>[3x]MDTKGRLVAGSHNRNEFVLINADETARVAVTELSGQICQICGDELEVTVNGEPFVACNECAFPVCRPCYEYERREGNQVCPQCKTRYKRIKGSPRVEGDEEEDDSDDLESEFDIGSVFSARLNYGSQVNGSVIHAPSEFDAASVASEIPLLTYGQEDVGISADKHALILPPFTARGKRVHPMPFPDSSVPVQPRPMDPKKDIAVYGYGSVAWKERMEDWKKKQSEKLQVVRHEGGKDSDELDDPDLPKMDEGRQPLWRKLPISSSRINPYRIIIVLRIAILCLFFHYRILHPVNDAYALWLTSVICEIWFAVSWIFDQFPKWSPILRETYLDRLSLRYEKEGKPSLLADIDVFVSTVDPMKEPPLITANTVLSILAVDYPVDK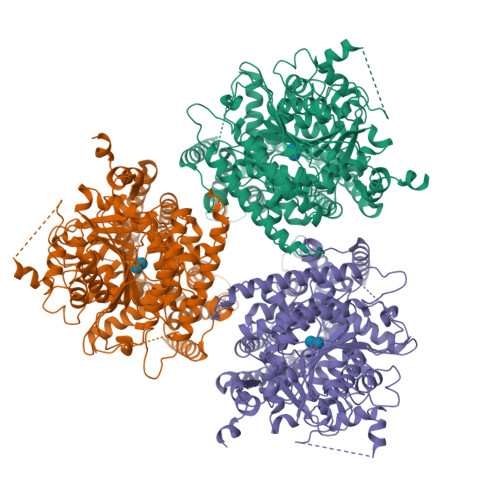VACYVSDDGAAMLTFEALSETSEFARKWVPFCKKFCIEPRAPEWYFAQKVDYLKDKVDATFIRERRAIKREYEEFKVRINALVALAQKVPEDGWTMQDGTPWPGNNVRDHPGMIQVFLGQNGVRDIEGNELPRLVYVSREKRPGYDHHKKAGAMNALVRVSAIITNAPYVLNVDCDHYINNSKALREAMCFMMDPTSGKKICYVQFPQRFDGIDRHDRYSNRNVVFFDINMKGLDGIQGPIYVGTGCVFRRQAFYGYDAPTSKKAPRKTCNCWPKWCCCLCCGSKKKKIKAKSSVKKKIKNKDDIKQMHALENIEEGIEGIDNEKSSLMSQSKFEKKFGQSSVFIASTLLEDGGVPKAASSATLLKEAIHVISCGYEDKTEWGKEVGWIYGSVTEDILTGFKMHCHGWRSVYCMPKRPAFKGSAPINLSDRLHQVLRWALGSVEIFFSRHCPIWYGYGGGLKSLERFSYINSVVYPLTSIPLIAYCALPAVCLLTGKFIVPEISNYASIIFMALFISIAATGILEMQWGGVGIHDWWRNEQFWVIGGASSHLFALFQGLLKVLAGVNTNFTVTSKAADDGEFADLYIFKWTSLLIPPLTLLIINIIGVIVGVSDAINNGYDSWGPLFGRLFFALWVIVHLYPFLKGVMGKQEGVPTIILVWAILLSSILTLLWVRINPFLAKSDVVLEICGLNCD(5S,7E,9E,11Z,14Z)-5-hydroxyicosa-7,9,11,14-tetraenoic 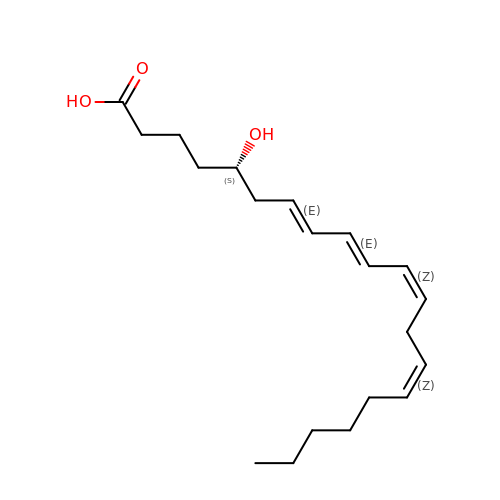acid | C20 H32 O3 | DVGDBDLZYCUGNU-LBIUVHPXSA-N>PQMTRENKAPNMSVRAQNVTVSNSRRRRRKNRKPRKQVEQATILKPQLLPGESVAPSGGRGTMDPPVHEICAQSIDPSEGAVGWFYKYMDPAGAVESGKALGEFSKVPDGLLRYSVDAEQRPIVTIECPTVSESDLPLDGKLWRVSFISFPAFRLNFIALANINNEALTLETRNTFIQTLNNITNWRDLGTGQWAQFAPGWYYSIYVLPNTYAMAEIGDRTDSVTQFRKVYKGITFEFNAPTLIDQGWWVGAHIPVKPQSETIPAAERFSAGSMTVSASNAIFQPSNTVARIVWSITPLPVATVALTTGTGGTNNTSGKFFSVEIDGNVNSVWTFTAPASILAEGEPFAEEGDTTSFSMTTITADTVVYSVSSSLTGSSVIVRGVTKGSGVSITPVTVGIDTEAVNRLSIEMPALTTEEVTTNVPKYEQFLCKESGGAYIVHYKMNNPVFEMTGEENFGGFQFHYPGYDPENNALGLRGIVDTFENNFSSAVVHFWGISQSATIVCKTYDGWEGTTNAGSTVGQFAHTGAEEEDEVVQLANRLQMELTGVYQADDN[4x];>FAGTVSALASIGLGLLGKSSATPSVIKGIAQQAVGAVQA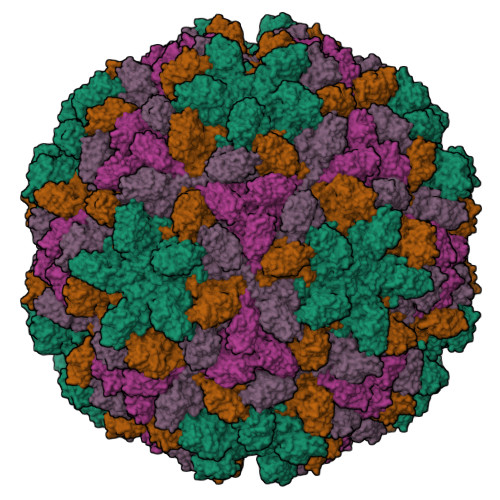NPGILEGAVKAIGSVGARLVGSIKARRARRRARRAK[4x]> MDAQYDISFADVEKAHINIRDSIHLTPVLTSSILNQLTGR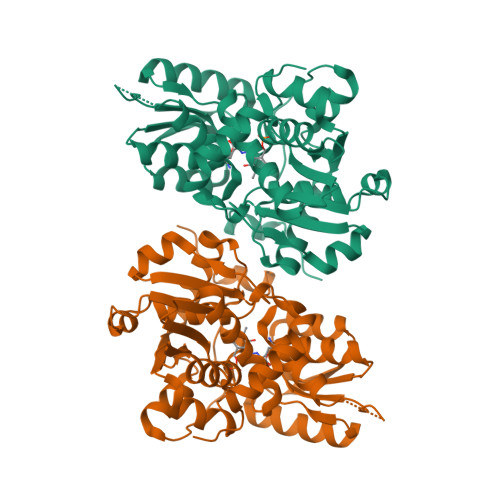NLFFKCELFQKTGSFKIRGALNAVRSLVPDALERKPKAVVTHSSGNHGQALTYAAKLEGIPAYIVVPQTAPDCKKLAIQAYGASIVYCEPSDESRENVAKRVTEETEGIMVHPNQEPAVIAGQGTIALEVLNQVPLVDALVVPVGGGGMLAGIAITVKALKPSVKVYAAEPSNADDCYQSKLKGKLMPNLYPPETIADGVKSSIGLNTWPIIRDLVDDIFTVTEDEIKCATQLVWERMKLLIEPTAGVGVAAVLSQHFQTVSPEVKNICIVLSGGNVDLTSSITWVKQAERPASYQSVSVHHHHHH> IINGEDCSPHSQPWQAALVMENELFCSGVLVHPQWVLSAAHCFQNSY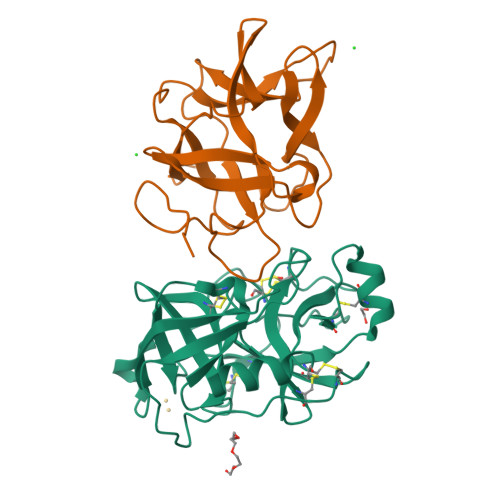TIGLGLHSLEADQEPGSQMVEASLSVRHPEYNRPLLANDLMLIKLDESVSESDTIRSISIASQCPTAGNSCLVSGWGLLANGRMPTVLQCVNVSVVSEEVCSKLYDPLYHPSMFCAGGGQDQKDSCNGDSGGPLICNGYLQGLVSFGKAPCGQVGVPGVYTNLCKFTEWIEKTVQA;> SSVVVDTNGQPVSNGADAYYLVPVSHGHAGLALAKIGNEAEPRAVVLDPHHRPGLPVRFESPLAINIIKESYFLNIKFGPSSSDSGVWDVIQQDPIGLAVKVTDTKSLLGPFKVEKEGEGYKIVYYPERGQTGLDIGLVHRNDKYYLAVKDGEPCVFKIRKATDE>[2x]GPMETAQYSTSKTPYSPQQDIRTYQPPPPGFTAVFTELVSRHGSRTPTKIDGADLLLQLWAKARDESELTSAGQDFGPTMESYRAAIQKVGLGQETGRGRQELQGMADRMQRRLPELFEKIKKDATPIAVVLSQQTGRIADTAKFFTARLGATDPALAPLIQQPVVDQDLLYFHKTERGKAYRDYLENDQRYQETVKRIKNRDGTRE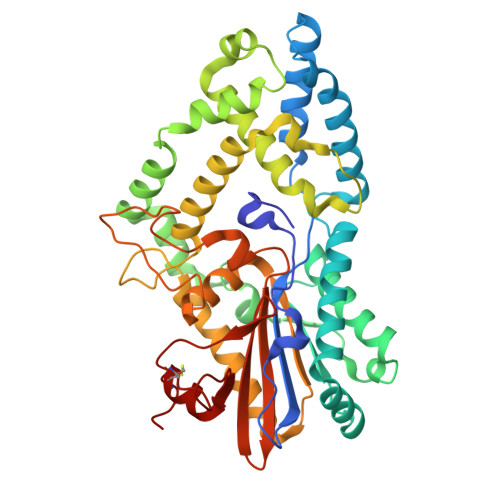AATDILKTIFTPAFVERMEPSAVTKAAQALYDLDAIAPDLSVEGNWHLDRFVPRHAAAWFASIDDAKSFYKKGPGFEGSDITFAMASILLDDFFKQAEAARAGKLGADLRFTHAEEIIPLAALMQLPGSEKQADPDEDYTYANNPWRGASVSPMAANLQWDIYRNGTTYLVRMLYQEKEIPFKPDCTPFTPGSHYYRLDELSRCFGRTAR We sought to develop a general computational method for de novo designing protein nanoparticles with geometries tailored to present antigens of interest, focusing specifically on the prefusion conformations of the trimeric viral glycoproteins HIV-1 Env (BG505 SOSIP), influenza hemagglutinin (H1 HA), and respiratory syncytial virus (RSV) F (DS-Cav1). In the first step, we de novo designed antigen-tailored trimers, featuring N termini geometrically matched to the C termini of the viral glycoproteins. In the second step, we generated tetrahedral, octahedral, and icosahedral two-component nanoparticles by designing secondary interfaces between a designed trimer (fusion component) and a de novo homo-oligomer (assembly component). This design approach yielded nanoparticles tailored to present 4, 8, or 20 copies of the viral glycoproteins in defined geometries.

As secondary assembly components were required to design our antigen-tailored nanoparticles, validated trimers were docked pairwise with de novo designed symmetric homo-oligomers to generate tetrahedral, octahedral, and icosahedral nanoparticle configurations using the TCdock program. Five designs comprising a panel of unique geometric configurations, T33_dn2, T33_dn5, T33_dn10, O43_dn18, and I53_dn5, ran as monodisperse particles of the predicted molecular mass by SEC-MALS and were further investigated by SAXS. The experimental solution scattering curves closely matched the scattering curves computed from the design models for all five designs (metrics in Table 1 and Figure 2—source data 1, bottom five designs). In order to obtain higher-resolution information, three designs, T33_dn10, O43_dn18, and I53_dn5, representing one nanoparticle from each targeted symmetry (T, O, I), were subjected to cryo-electron microscopy (cryo-EM). The final resolutions of the reconstructed maps for the T33_dn10, O43_dn18, and I53_dn5 nanoparticles were 3.9, 4.5, and 5.3 Å, respectively. There is less evidence of flexibility in T33_dn10 and O43_dn18, in agreement with the higher final map resolution for these nanoparticles. Nanoparticle design models were relaxed into the corresponding EM maps by applying multiple rounds of Rosetta relaxed refinement and manual refinement in Coot to generate the final structures. Overall, the refined structures show excellent agreement with the corresponding Rosetta design models. Backbone r.m.s.d. values estimated for the asymmetric unit (consisting of a single subunit of component A and component B) were 0.65, 0.98, and 1.3 Å for T33_dn10, O43_dn18, and I53_dn5, respectively. The self-assembling cores of the antigen-fused T33_dn2, T33_dn10, and I53_dn5 nanoparticles were very similar to the NS-EM maps of the unmodified nanoparticles (at least to the resolution limits of NS-EM), demonstrating that fusion of the BG505 SOSIP trimer did not induce any major structural changes to the underlying nanoparticle scaffolds.

> MGEEAELAYLLGELAYKLGEYRIAIRAYRIALKRDPNNAEAWYNLGNAYYKQGDYDEAIEYYQKALELDPNNAEAWYNLGNAYYKQGDYDEAIEYYEKALELDPENLEALQNLLNAMDKQG;> MIEEVVAEMIDILAESSKKSIEELARAADNKTTEKAVAEAIEEIARLATAAIQLIEALAKNLASEEFMARAISAIAELAKKAIEAIYRLADNHTTDTFMARAIAAIANLAVTAILAIAALASNHTTEEFMARAISAIAELAKKAIEAIYRLADNHTTDKFMAAAIEAIALLATLAILAIALLASNHTTEKFMARAIMAIAILAAKAIEAIYRLADNHTSPTYIEKAIEAIEKIARKAIKAIEMLAKNITTEEYKEKAKKIIDIIRKLAKMAIKKLEDNRTLEHHHHHH(2S,3S)-3-methyl-2-[[2-methyl-3-oxidanyl-5-(phosphonooxymethyl)pyridin-4-yl]methylamino]pentanoic acid | C14 H23 N2 O7 P | 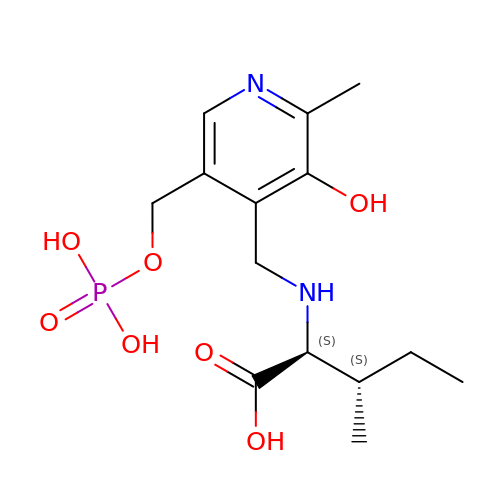GZZDWFDWHXPWJK-UFBFGSQYSA-N>[4x]MPVIAANDGCLTVFNMFTTDTIDGQRELLKEMRDII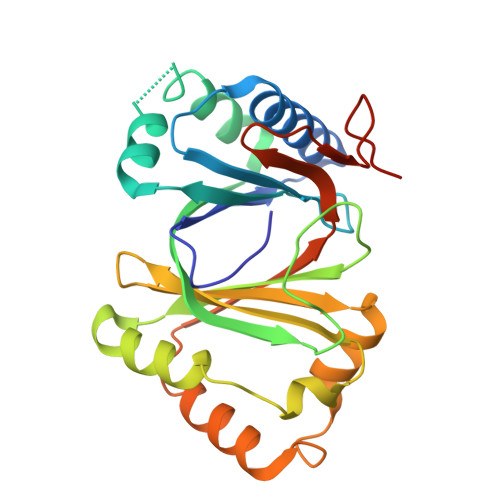DNGNFTGWRSSTLHAGQDEHGTANYIQWRSLADLEARYAGEGYKNNTVPLFKQISTSVHLLKTEVVFSQHHPDLPRIEISPERDDYTVIIVMDVAAQDQAALVQVLGRPDEWIKTVPGYLSHALCRGIDGTFVVLYAQWESKERYDAFHTMPESARPQAVREQRAFTDTLITARRSNTYRVVHTRSAGSPAVSIMNQEGTWQARATSRP[4-(5-bromanyl-3-methyl-pyridin-2-yl)piperazin-1-yl]-[3-(2-chlorophenyl)-5-methyl-1,2-oxazol-4-yl]methanone 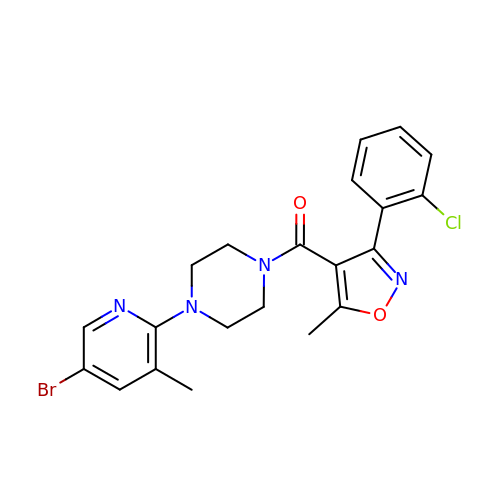| C21 H20 Br Cl N4 O2 | FJRSKYVUWHZUJT-UHFFFAOYSA-N>[2x]MKVGIVGSGMVGSATAYALALLGVAREVVLVDLDRKLAQAHAEDILHATPFAHPVWVWAGSYGDLEGARAVVLAAGVAQRPGETRLQLLDRNAQVFAQVVPRVLEAAPEAVLLVATNPVDVMTQVAYALSGLPPGRVVGSGTILDTARFRALLAEYLRVAPQSVHAYVLGEHGDSEVLVWSSAQVGGVPLLEFAEARGRALSPEDRARIDEGVRRAAYRIIEGKGATYYGIGAGLARLVRAILTDEK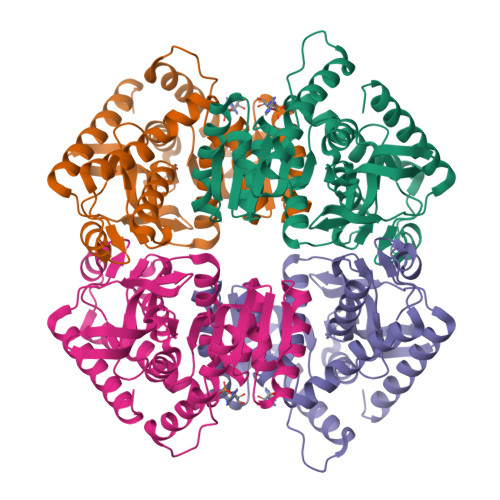GVYTVSAFTPEVAGVLEVSLSLPRILGAGGVAGTVYPSLSPEERAALRRSAEILKEAAFALGF> MREYKLVVLGSGGVGKSALTVQFVQGIFVEKYDPTIEDSYRKQVEVDAQQCMLEILDTAGTEQFTAMRDLYMKNGQGFALVYSITAQSTFNDLQDLREQILRVKDTDDVPMILVGNKCDLEDERVV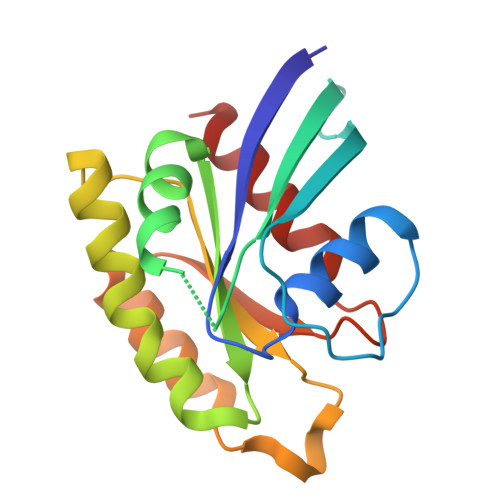GKEQGQNLARQWNNCAFLESSAKSKINVNEIFYDLVRQINR N-ACETYL-D-PROLINE | C7 H11 N O3 | 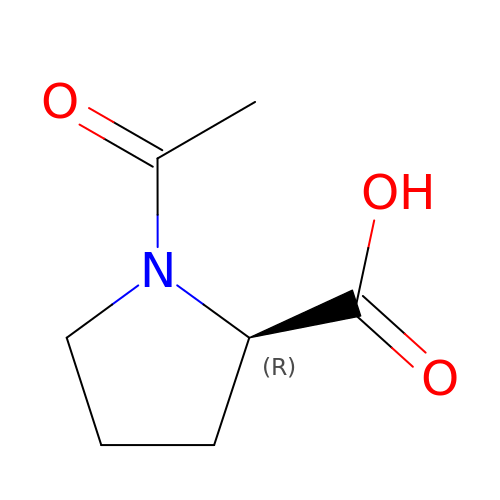GNMSLDIYJOSUSW-ZCFIWIBFSA-N Here, we show that Yersinia pseudotuberculosis secretes an effector, CccR, that can act both as a toxin and as a transcriptional factor. CccR contains an N-terminal FIC domain and a C-terminal DNA-binding domain. In E. coli cells, the FIC domain of CccR AMPylates the cell division protein FtsZ, inducing cell filamentation and growth arrest. In Y. pseudotuberculosis cells, CccR inhibits its own expression by binding through its DNA-binding domain to the cccR promoter, and affects the expression of other genes through unclear mechanisms.

To understand the biological role of CccR at the molecular level, we determined its crystal structure using the single-wavelength anomalous method (SAD) at a 2.78 Å resolution. The crystallographic asymmetric unit contains two molecules of CccR assembled into a butterfly-shaped homodimer. The two CccR molecules within the homodimer are nearly identical to each other, as they were superimposed with a root-mean-square deviation value of 0.593 Å over 340 Cα atoms. Dimerization is mainly mediated by interactions formed between the α1 helices and the N-terminal loops of each CccR monomer. Specifically, the side chain of residue K175 from the α5-α6 loop of one monomer forms a salt bridge with the side chain of residue D22 from the α1 helix of the other monomer. AUC analysis indicated that simultaneous substitution of N13 and K175 with alanine abolishes dimerization. The 26-bp spacer between binding boxes is unusually large but is compatible with the 70.2 Å separation between DNA-binding helices observed in the CccR apo structure. As a Class II FIC protein, CccR contains an N terminal αinh (S59ARIEG). The crystal structure of CccR shows S59 and E63 form a stable hydrogen bond with R203 to prevent binding of the ATP substrate for modification.

>MPKFNHYDLALLNPSFDSPLVDALTELELLRHLRLETDVHPLLFAQLKSIFHMLESLGSARIEGNHTTLADYVESKVEGAEDSTDQLKEIGNIEHAMNFIDEHLHAGEDITEYFVRELHAMTVNGLEREGDKTPGAYRSHGVSIAQSTHLPPEFIHVPAYMQELVGFMNRADAPKYDLMKVALAHHRFGWIHPFGNGNGRTVRLLTYSLLIKYGFNVKTSGRVLNPTAVFCNDRERYYSMLAEADTGAVEGLEQWCLYVLTGISAELKKVDKLSDLHFLNSKVLYPALEYSKGRGVINETESKILKRTISQGTVKTSDLKEVLPGLKPAQITYQIGKLVDRGLLQPVEVGSRIYTAGFSKSDLMRGVIHALRKEGFIPDF[2x]>[16x]MKKFNIKSLTLLIVLLPLIVNANNIDSHLLEQNDIAKYVAQSDTVGSFFERFSALLNYPIVVSKQAAKKRISGEFDLSNPEEMLEKLTLLVGLIWYKDGNALYIYDSGELISKVILLENISLNYLIQYLKDANLYDHRYPIRGNISDKTFYISGPPALVELVANTATLLDKQVSSIGTDKVNFGVIKLKNTFVSDRTYNMRGEDIVIPGVATVVERLLNNGKALSNRQAQNDPMPPFNITQKVSEDSNDFSFSSVTNSSILEDVSLIAYPETNSILVKGNDQQIQIIRDIITQLDVAKRHIELSLWIIDIDKSELNNLGVNWQGTASFGDSFGASFNMSSSASISTLDGNKFIASVMALNQKKKANVVSRPVILTQENIPAIFDNNRTFYVSLVGERNSSLEHVTYGTLINVIPRFSSRGQIEMSLTIEDGTGNSQSNYNYNNENTSVLPEVGRTKISTIARVPQGKSLLIGGYTHETNSNEIISIPFLSSIPVIGNVFKYKTSNISNIVRVFLIQPREIKESSYYNTAEYKSLISEREIQKTTQIIPSETTLLEDEKSLVSYLNY;>MLSDMSLIATLSFFTLLPFLVAAGTCYIKFSIVFVMVRNALGLQQVPSNMTLNGIALIMALFVMKPIIEAGYENYLNGPQKFDTISDIVRFSDSGLMEYKQYLKKHTDLELARFFQRSEEENADLKSAENNDYSLFSLLPAYALSEIKDAFKIGFYLYLPFVVVDLVISSILLALGMMMMSPITISVPIKLVLFVALDGWGILSKALIEQYINIPA[5x];> MDISSWFESIHVFLILLNGVFFRLAPLFFFLPFLNNGIISPSIRIPVIFLVASGLITSGKVDIGSSVFEHVYFLMFKEIIVGLLLSFCLSLPFWIFHAVGSIIDNQRGATLSSSIDPANGVDTSELAKFFNLFSAVVFLYSGGMVFILESIQLSYNICPLFSQCSFRISNILTFLTLLASQAVILASPVMIVLLLSEVLLGVLSRFAPQMNAFSVSLTIKSLLAIFIIFICSSTIYFSKVQFFLGEHKFFTNLFVR;>MSDIVYMGNKALYLILIFSLWPVGIATVIGLSIGLLQTVTQLQEQTLPFGIKLIGVSISLLLLSGWYGEVLLSFCHEIMFLIKSGV[4x];> MANKTEKPTPKKLKDAAKKGQSFKFKDLTTVVIILVGTFTIISFFSLSDVMLLYRYVIINDFEINEGKYFFAVVIVFFKIIGFPLFFCVLSAVLPTLVQTKFVLATKAIKIDFSVLNPVKGLKKIFSIKTIKEFFKSILLLIILALTTYFFWINDRKIIFSQVFSSVDGLYLIWGRLFKDIILFFLAFSILVIILDFVIEFILYMKDMMMDKQEIKREYIEQEGHFETKSRRRELHIEILSEQTKSDIRNSKLVVMNPTHIAIGIYFNPEIAPAPFISLIETNQCALAVRKYANEVGIPTVRDVKLARKLYKTHTKYSFVDFEHLDEVLRLIVWLEQVENTH;>MNYIYPVNQVDIIKASDFQSQEISSLEDVVSAKYSDIKMDTDIQVSQIMEMVSNPESLNPESLAKLQTTLSNYSIGVSLAGTLARKTVSAVETLLKS[6x];>[28x]MASWSHPQFEKIEGRMSVTVPNDDWTLSSLSETFDDGTQTLQGELTLALDKLAKNPSNPQLLAEYQSKLSEYTLYRNAQSNTVKVIKDVDAAIIQNFR;>[24x]MIRYKGFILFLLLMLIGCEQREELISNLSQRQANEIISVLERHNITARKVDGGKQGISVQVEKGTFASAVDLMRMYDLPNPERVDISQMFPTDSLVSSPRAEKARLYSAIEQRLEQSLVSIGGVISAKIHVSYDLEEKNISSKPMHISVIAIYDSPKESELLVSNIKRFLKNTFSDVKYENISVILTPKEEYVYTNVQPVKEVKSEFLTNEVIYLFLGMAVLVVILLVWAFKTGWFKRNKI

The type III secretion system (T3SS) is a large, transmembrane protein machinery used by various pathogenic gram‐negative bacteria to transport virulence factors into the host cell during infection. The T3SS is a large, syringe‐shaped, membrane‐spanning, multimegadalton protein machinery. While the needle is a helical complex composed of a single protein (MxiH in Shigella [SctF in the unified nomenclature; Hueck, 1998]) (Demers et al., 2013), the basal body comprises multiple different proteins, either forming membrane‐associated periplasmic rings (MxiD[SctC], MxiG[SctD], MxiJ[SctJ] in Shigella) or the pseudohelical structure of the export apparatus core (SpaP[SctR], SpaQ[SctS], SpaR[SctT], and SpaS[SctU] in Shigella; Blocker et al., 2001; Lunelli et al., 2020). Here, we combined cryo‐electron microscopy, cross‐linking mass spectrometry, and integrative modeling to determine the structure of the T3SS needle complex from Shigella flexneri.

Regions inside the needle complex, which do not exhibit any symmetry, could be resolved up to 3.6 Å in a map without imposed symmetry (“C1 map”), enabling us to build the de novo atomic model of the proximal needle end and the export apparatus. As in the previously published structures of the Shigella export apparatus (Johnson et al., 2019; Lunelli et al., 2020), our updated cryo‐EM structure includes five SpaP[SctR], four SpaQ[SctS], and one SpaR[SctT] subunit. In addition, we were able to model the N‐terminal domain of the SpaS[SctU] subunit, which was not resolved in our previous reconstruction and also not resolved in the published structures of the Salmonella T3SS. The SpaP[SctR] and SpaR[SctT] form the core of the complex, whereas the SpaQ[SctS] and SpaS[SctU] subunits form smaller helical hairpins that decorate the outer surface. The transport channel at this side is closed by the side chains of the residues F213 of SpaR[SctT] and M178, M179 of the five SpaP[SctR] subunits, while the flanking M177 and M180 do not extend their side chains in the channel lumen. Although we do not observe the long loop, the N‐terminal domain of SpaS[SctU] has a similar topology to the flagellar FlhB[SctU]. The improved C1 map presented here clearly shows that six MxiI[SctI] subunits assemble into a single helical turn before being continued by the needle protein MxiH[SctF]. The six MxiI[SctI] subunits build the first turn of an upward spiral on the distal side of the export apparatus creating interfaces with all SpaP[SctR] (SpaP[SctR]1–5) and the only SpaR[SctT] subunit of the complex. The β‐strand augments a β‐sheet of the N1 domain of MxiD[SctC] (S112‐V116), anchoring the needle‐ and export apparatus structure within the basal body.4-{[(3S)-3-(5-methyl-2,4-dioxo-3,4-dihydropyrimidin-1(2H)-yl)piperidin-1-yl]methyl}-2-[3-(trifluoromethyl)phenoxy]benzoic acid | C25 H24 F3 N3 O5 | 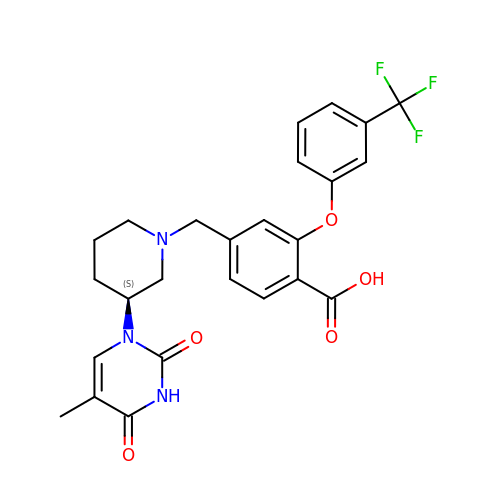SLYIQORXPGMWOF-SFHVURJKSA-N> MATDVAQGPNGRALAESMNPDLLSAIQQHISIERY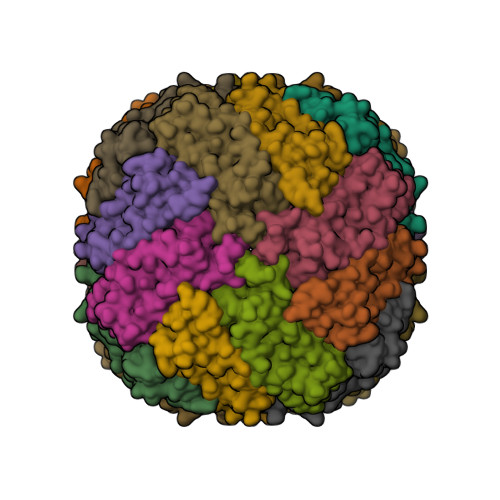ASVTYLAMSIWCAERELAGFYQFFDGEAKDEQSHAVHFTQYLIARSQSNDLQTLDAPRQNWDSLASLMATAFQMEADTTSSIQSVYALAERNSDTRTTVFLDPLIAAQIQSEDQFAYLLGRVKFANGDPTALLVIDNELRAGQTQRG> MSTRKIFDSEEQSFIRLVDKFYLGLSLTKLCAQSCNL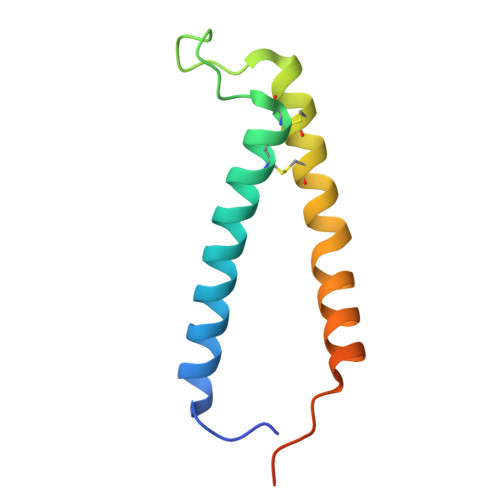LRNDISGSALTQKEKDCLSICYNNIEKTQSAFYAKVKTTMNLPAVEDDGEEGGDDE> MWPVD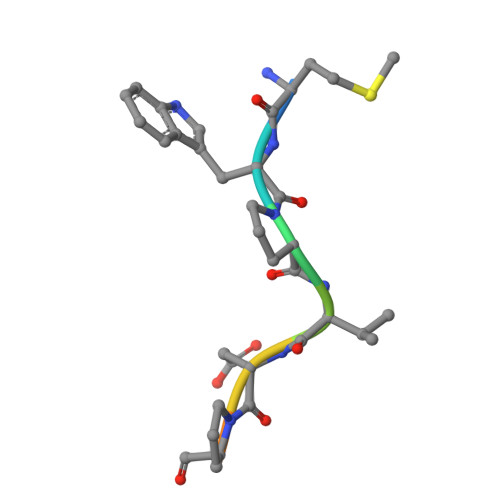PNIE>MTFEEKLSKIYNEIANEISSMIPVEWEKVYTMAYIDDGGGEVFFNYTKPGSDDLNYYTNIPKEYNISVQVFDDLWMDLYDLFEELRDLFKEEDLEPWTSCEFDFTREGELKVSFDYIDWINSEFGQIGRQNYYKYRKFGILPETEYEINKVKEIEQYIKELE[2x]

Toxin EsaD secreted by some S. aureus strains through the type VII secretion system (T7SS) specifically kills those strains lacking the antitoxin EsaG. EsaD is a toxin secreted in a T7SS machinery-dependent manner by S. aureus. Here we report the structures of EsaG, the nuclease domain of EsaD and their complex, which together reveal an inhibition mechanism that relies on significant conformational change of the toxin. The major contribution of this study is the discovery of an inhibitory mechanism in the toxin-antitoxin module that is based on a significant structural deformation of the toxin, where the central β-sheet of the nuclease domain of EsaD is split by EsaG into two fragments.

To investigate whether EsaG contains an IDR domain as most of the other type II antitoxins, we determined the crystal structure of full-length EsaG at a resolution of 2.30 Ǻ. There are two EsaG molecules in the asymmetric unit, which interact with each other in a 2-fold symmetry. Even though gel-filtration experiments indicated a dimer state, chemical cross-linking of EsaG using an amine-specific crosslinking reagent EGS (ethylene glycol bis(succinimidyl succinate)) yielded no cross-linked product. Density gradient centrifugation analysis also supported a monomer form. The structure of EsaG contains a principle four-stranded β-sheet sandwiched by αA’, αB’ and αC’ from one side and αD’ and αE’ from the other side. We noticed that, except for three residues (G50–S51 on loopβ2’-αB’ and E162 on the C-terminus), electron densities were observed for all the other residues of EsaG. Similarly, BH3703 is also well structured with only three residues in the C-terminus missing. This suggests the absence of IDRs in EsaG-like antitoxins and, therefore, a distinct toxin inhibition mechanism in Gram-positive bacteria. Except for subtle movements in some loops, no obvious conformational change happens on EsaG upon EsaDc binding, further supporting the absence of IDR in the inhibition process. In contrast, we didn’t observe any disorder-to-order conversion of the antitoxin EsaG in the structures of EsaG and EsaDc-EsaG complex.>MNTVRSEKDSMGAIDVPADKLWGAQTQRSLEHFRISTEKMPTSLIHALALTKRAAAKVNEDLGLLSEEKASAIRQAADEVLAGQHDDEFPLAIWQTGSGTQSNMNMNEVLANRASELLGGVRGMERKVHPNDDVNKSQSSNDVFPTAMHVAALLALRKQLIPQLKTLTQTLNEKSRAFADIVKIGRTHLQDATPLTLGQEISGWVAMLEHNLKHIEYSLPHVAELALGGTAVGTGLNTHPEYARRVADELAVITCAPFVTAPNKFEALATCDALVQAHGALKGLAASLMKIANDVRWLASGPRCGIGEISIPENEPGSSIMPGAVNPTQCEALTMLCCQVMGNDVAINMGGASGNFELNVFRPMVIHNFLQSVRLLADGMESFNKHCAVGIEPNRERINQLLNESLMLVTALNTHIGYDKA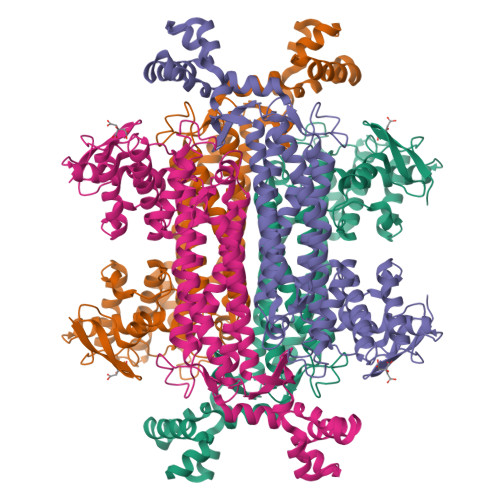AEIAKKAHKEGLTLKAAALALGYLSEAEFDSWVRPEQMVGSMKAGRHHHHH[2x]> GEIQWVKPNKETGRLNINGPTRTKLEPSVFHDVFEGNKEPAVLHSKDPRLEVDFEQALFSKYVGNTLYEPDEYIKEAALHYANQLKQLDIDTSQMSMEEACYGTENLEAIDLHTSAGYPYSALGIKKRDILDSTTRDVSKMKF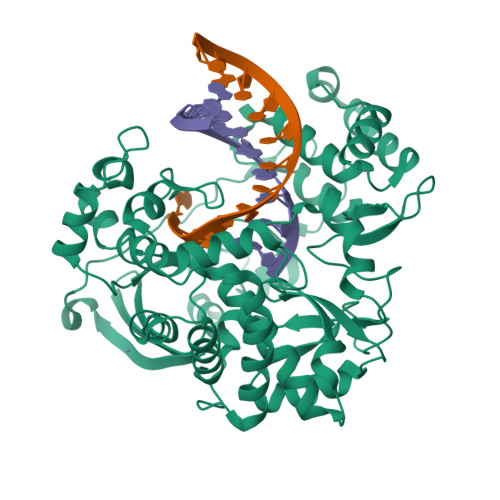YMDKYGLDLPYSTYVKDELRSIDKIKKGKSRLIEASSLNDSVYLRMTFGHLYETFHANPGTVTGSAVGCNPDTFWSKLPILLPGSLFAFDYSGYDASLSPVWFRALELVLREIGYSEEAVSLVEGINHTHHVYRNKTYCVLGGMPSGCSGTSIFNSMINNIIIRALLIKTFKGIDLDELNMVAYGDDVLASYPFPIDCLELARTGKEYGLTMTPADKSPCFNEVNWDNATFLKRGFLPDEQFPFLIHPTMPMKEIHESIRWTKDARNTQDHVRSLCLLAWHNGKQEYEKFVSAIRSVPVGKALAIPNYENLRRNWLELFHHHHHH>[2x]QTITVWSWQTGPELQDVKQIAAQWAKAHGDKVIVVDQSSNPKGFQFYATAARTGKGPDVVFGMPHDNNGVFAEEGLMAPVPSGVLNTGLYAPNTIDAIKVNGTMYSVPVSVQVAAI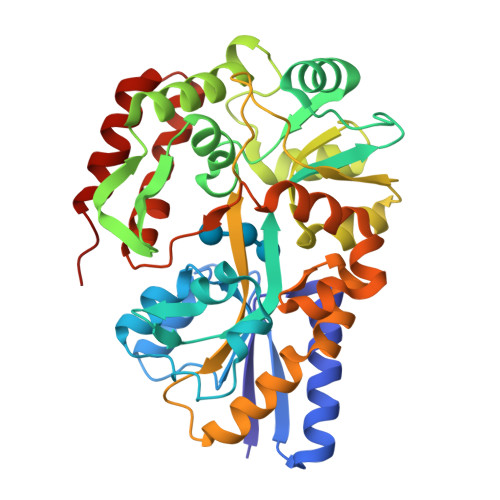YYNKKLVPQPPQTWAEFVKDANAHGFMYDQANLYFDYAIIGGYGGYVFKDNNGTLDPNNIGLDTPGAVQAYTLMRDMVSKYHWMTPSTNGSIAKAEFLAGKIGMYVSGPWDTADIEKAKIDFGVTPWPTLPNGKHATPFLGVITAFVNKESKTQAADWSLVQALTSAQAQQMYFRDSQQIPALLSVQRSSAVQSSPTFKAFVEQLRYAVPMPNIPQMQAVWQAMSILQNIIAGKVSPEQGAKDFVQNIQKGIMA> MTERTLVLIKPDGIERQLIGEIISRIERKGLTIAALQLRTVSAELASQHYAEHEGKPFFGSLLEFITSGPVVAAIVEGTRAIAAVRQLAGGTNPVQAAAPGTIRGDFALETQFNLVHG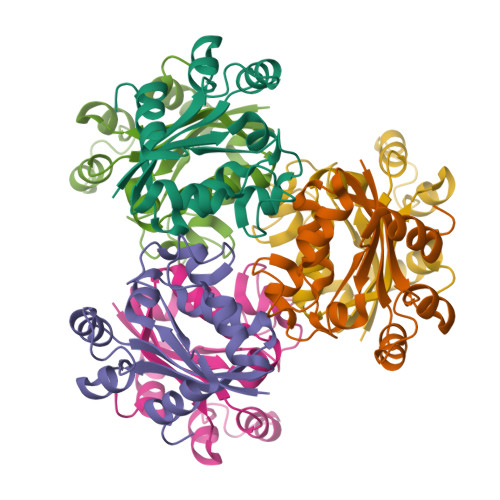SDSAESAQREIALWFPGA> YLQKPMYEVQWKVVEEINGNNYVYIDPTQLPYDHKWEFPRNRLSFGKTLGAGAFGKVVEATAY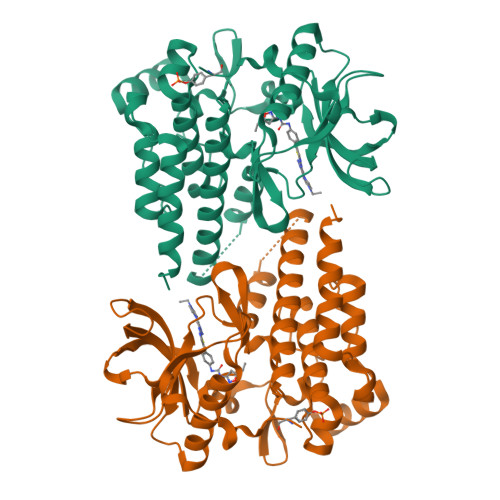GLIKSDAAMTVAVKMLKPSAHLTEREALMSELKVLSYLGNHMNIVNLLGACTIGGPTLVITEYCCYGDLLNFLRRKRDSFICSKTSPAIMEDDELALDLEDLLSFSYQVAKGMAFLASKNCIHRDLAARNILLTHGRITKICDFGLARDIKNDSNYVVKGNARLPVKWMAPESIFNCVYTFESDVWSYGIFLWELFSLGSSPYPGMPVDSKFYKMIKEGFRMLSPEHAPAEMYDIMKTCWDADPLKRPTFKQIVQLIEKQISESTNHI>LRNRATDLDARMHDGTTPLILAARLALEGMLEDLINSHADVNAVDDLGKSALHWAAAVNNVDAAVVLLKNGANKDMQNNKEETPLFLAAREGSYETAKVLLDHFANRDITDHMDRLPRDIAQERMHHD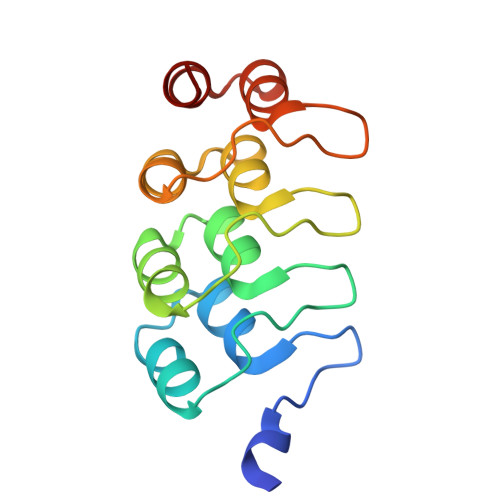IVRLLDE[2x]>PISPIETVPVKLKPGMDGPKVKQWPLTEEKIKALVEICTEMEKEGKISKIGPENPYNTPVFAIKKKDSTKWRKLVDFRELNKRTQDFWEVQLGIPHPAGLKKKKSVTVLDVGDAYFSVPLDEDFRKYTAFTIPSINNETPGIRYQYNVLPQGWKGSPAIFQSSMTKILEPFKKQNPDIVIYQYMDDLYVGSDLEIGQHRTKIEELRQHLLRWGLTTPDKKHQKEPPFLWMGYELHPDKWTVQPIVLPEKDSWTVNDIQKLVGKLNWASQIYPGIKVRQLSKLLRGTKALTEVIPLTEEAELELAENREILKEPVHGVYYDPSKDLIAEIQKQGQGQWTYQIYQEPFKNLKTGKYARMRGAHTNDVKQLTEAVQKITTESIVIWGKTPKFKLPIQKETWETWWTEYWQATWIPEWEFVNTPPLVKLWYQLEKEPIVGAETFYVDGAANRETKLGKAGYVTNKGRQKVVPLTNTTNQKTELQAIYLALQDSGLEVNIVTNSQYALGIIQAQPDKSESELVNQIIEQLIKKEKVYLAWVPAHKGIGGNEQVDKLVSAG[2x];>GPISPIETVPVKLKPGMDGPKVKQW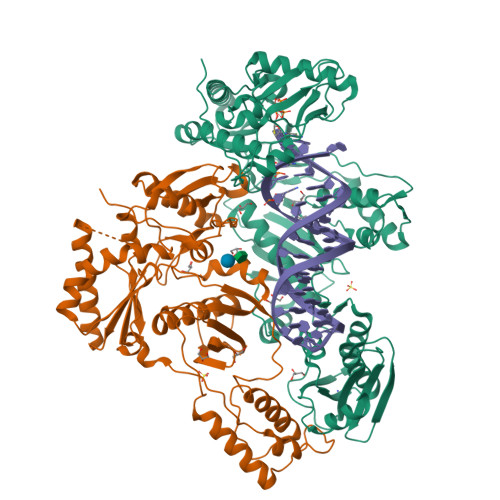PLTEEKIKALVEICTEMEKEGKISKIGPENPYNTPVFAIKKKDSTKWRKLVDFRELNKRTQDFWEVQLGIPHPAGLKKKKSVTVLDVGDAYFSVPLDEDFRKYTAFTIPSINNETPGIRYQYNVLPQGWKGSPAIFQSSMTKILEPFKKQNPDIVIYQYMDDLYVGSDLEIGQHRTKIEELRQHLLRWGLTTPDKKHQKEPPFLWMGYELHPDKWTVQPIVLPEKDSWTVNDIQKLVGKLNWASQIYPGIKVRQLSKLLRGTKALTEVIPLTEEAELELAENREILKEPVHGVYYDPSKDLIAEIQKQGQGQWTYQIYQEPFKNLKTGKYARMRGAHTNDVKQLTEAVQKITTESIVIWGKTPKFKLPIQKETWETWWTEYWQATWIPEWEFVNTPPLVKLWYQ[2x]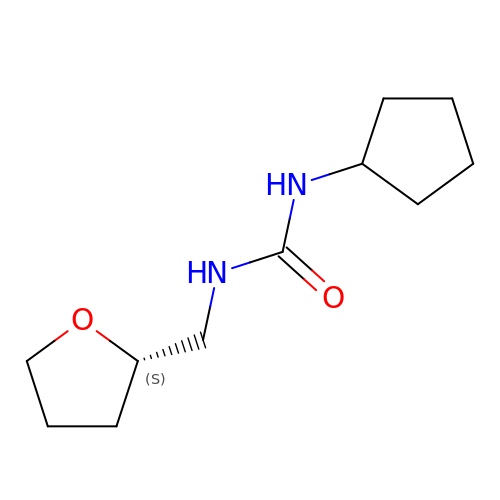1-cyclopentyl-3-[[(2~{S})-oxolan-2-yl]methyl]urea | C11 H20 N2 O2 | GZCFMEFTVSKHDE-JTQLQIEISA-N>[3x]MAAPMTPAARPEDYEAALNAALADVPELARLLEIDPYLKPYAVDFQRRYKQFSQILKNIGENEGGIDKFSRGYESFGVHRCADGGLYCKEWAPGAEGVFLTGDFNGWNPFSYPYKKLDYGKWELYIPPKQNKSVLVPHGSKLKVVITSKSGEILYRISPWAKYVVREGDNVNYDWIHWDPEHSYEFKHSRPKKPRSLRIYESHVGISSHEGKVASYKHFTCNVLPRIKGLGYNCIQLMAIMEHAYYASFGYQITSFFAASSRYGSPEELQELVDTAHSMGIIVLLDVVHSHASKNSADGLNMFDGTDSCYFHSGPRGTHDLWDSRLFAYSSWEVLRFLLSNIRWWLEEYRFDGFRFDGVTSMLYHHHGVGQGFSGDYSEYFGLQVDEDALTYLMLANHLVHTLCPDSITIAEDVSGMPALCSPISQGGGGFDYRLAMAIPDKWIQLLKEFKDEDWNMGDIVYTLTNRRYLEKCIAYAESHDQALVGDKSLAFWLMDAEMYTNMSVLTPFTPVIDRGIQLHKMIRLITHGLGGEGYLNFMGNEFGHPEWLDFPRKGNNESYHYARRQFHLTDDDLLRYKFLNNFDRDMNRLEERYGWLAAPQAYVSEKHEGNKIIAFERAGLLFIFNFHPSKSYTDYRVGTALPGKFKIVLDSDAAEYGGHQRLDHSTDFFSEAFEHNGRPYSLLVYIPSRVALILQNVDLPN

GBE (also known as 1,4-glucan:1,4-glucan 6-glucanotransferase) transfers α-1,4-linked glucose units from the outer ‘non-reducing’ end of a growing glycogen chain into an α-1,6 position of the same or neighbouring chain, thereby creating glycogen branches. Together GYS and GBE define the globular and branched structure of glycogen, which increases its solubility by creating a hydrophilic surface and regulates its synthesis by increasing the number of reactive termini for GYS-mediated chain elongation. Almost all sequence-annotated branching enzymes, including those from diverse organisms, belong to the GH13 family of glycosyl hydrolases (also known as the α-amylase family) and fall either into subfamily 8 (eukaryotic GBEs) or subfamily 9 (prokaryotic GBEs). In several GH13 enzymes, this constellation of three acidic residues functions as the nucleophile (Asp357, hGBE1 numbering hereinafter), proton donor (Glu412) and transition state stabilizer (Asp481) in the active site.

Interrogation of several N- and C-terminal boundaries in this expression system yielded a soluble and crystallisable polypeptide for hGBE1 from aa 38–700 (hGBE1trunc). Inspection of the asymmetric unit content as well as symmetry-related protomers did not reveal any stable oligomer arrangements, consistent with GBE1 being a monomer in size-exclusion chromatography (data not shown), similar to most GH13 enzymes. hGBE1 is an elongated molecule (longest dimension >85 Å) composed of four structural regions: the N-terminal helical segment (aa 43–75), a carbohydrate-binding module 48 (CBM48; aa 76–183), a central catalytic core (aa 184–600) and the C-terminal amylase-like barrel domain (aa 601–702). The hGBE1 active site is a prominent surface groove at the (βα)6-barrel that could bind a linear glucan chain via a number of subsites (left), each binding a single glucose unit. A region of GBE-unique sequences (aa 405–443), rich in Gly/Ala residues, has been identified based on alignment with GH13 sequences. This region, replaced in amylolytic enzymes by sequence insertions and bulkier residues, maps onto a hGBE1 surface that is proximal to the ‘+1, +2 …’ subsites, and to the β4-α4 loop that is disordered in hGBE1 but adopts different conformations in the O. sativa and M. tuberculosis structures (right). We posit that this surface region, unique to branching enzymes, facilitates access to the active site by an incoming glucan acceptor chain. Tyr329 is a surface-exposed residue in the catalytic domain and confers stability to the local environment by interacting with the hydrophobic residues Phe327, Val334, Leu338, Met362 and Ala389. Additionally, the tyrosyl hydroxyl group hydrogen bonds with the His289 backbone oxygen (left). Mutation of Tyr329 to the smaller amino acid serine (Ser329mutant) likely removes these interactions (right) and creates a solvent accessible cavity within this hydrophobic core, both of which could lead to destabilized protein.>[12x]MSLKIIDFRLRPPAMGFLNARIYTRPDIRNRFTRQLGFEPAPSAEEKSLELMFEEMAAAGIEQGVCVGRNSSVLGSVSNADVAAVAKAYPDKFHPVGSIEAATRKEAMAQMQEILDL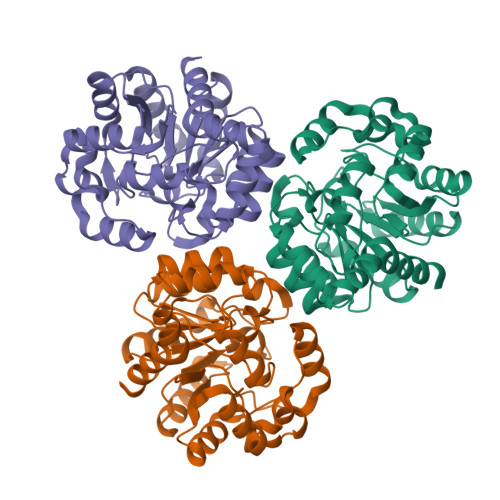GIRIVNLEPGVWATPMHVDDRRLYPLYAFCEDNGIPVIMMTGGNAGPDITYTNPEHIDRVLGDFPDLTVVSSHGNWPWVQEIIHVAFRRPNLYLSPDMYLYNLPGHADFIQAANSFLADRMLFGTAYPMCPLKEYTEWFLTLPIKPDAMEKILHGNAERLLAQAGREGHHHHHH>MKP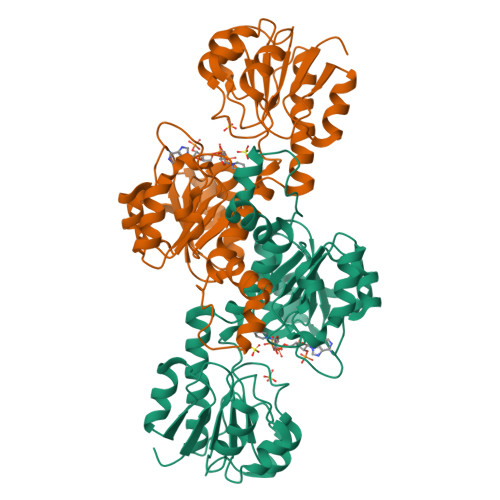KVFITREIPEVGIKMLEDEFEVEVWGDEKEIPREILLKKVKEVDALVTMLSERIDKEVFENAPKLRIVANYAVGYDNIDIEEATKRGIYVTNTPDVLTDATADLAFALLLATARHVVKGDRFVRSGEWKKRGVAWHPKWFLGYDVYGKTIGIIGLGRIGQAIAKRAKGFNMRILYYSRTRKEEVERELNAEFKPLEDLLRESDFVVLAVPLTRETYHLINEERLKLMKKTAILINIARGKVVDTNALVKALKEGWIAGAGLDVFEEEPYYNEELFKLDNVVLTPHIGSASFGAREGMAELVAKNLIAFKRGEIPPTLVNREVIKIRKPGFE[6x]> RVADTVGTGPTNSEAIPALTAAETGHTSQVVPGDTMQTRHVKNYHSRSESTIENFLCRSACVYFTEYENSGAKRYAEWVLTPRQAAQLRRKLEFFTYVRFDLELTFVITSTQQPSTTQNQDAQILTHQIMYVPPGGPVPDKVDSYVWQTSTNPSVFWTEGNAPPRMSIPFLSIGNAYSNFYDGWSEFSRNGVYGINTLNNMGTLYARHVNAGSTGPIKSTIRIYFKPKHVKAWIPRPPRLCQYEKAKNVNFQPSGVTTTRQSITTMTN;> GYSDRARSITLGNSTITTQECANVVVGYGVWPDYLKDSEATAEDQPTQPDVATCRFYTLDSVQWQKTSPGWWWKLPDALSNLGLFGQNMQYHYLGRTGYTVHVQCNASKFHQGCLLVVCVPEAEMGCATLDNTPSSAELLGGDSAKEFADKPVASGSNKLVQRVVYNAGMGVGVGNLTIFPHQWINLRTNNSATIVMPYTNSVPMDNMFRHNNVTLMVIPFVPLDYCPGSTTYVPITVTIAPMCAEYNGLRLAGHQ;> GLPTMNTPGSCQFLTSDDFQSPSAMPQYDVTPEMRIPGEVKNLMEIAEVDSVVPVQNVGEKVNSMEAYQIPVRSNEGSGTQVFGFPLQPGYSSVFSRTLLGEILNYYTHWSGSIKLTFMFCGSAMATGKFLLAYSPPGAGAPTKRVDAMLGTHVVWDVGLQS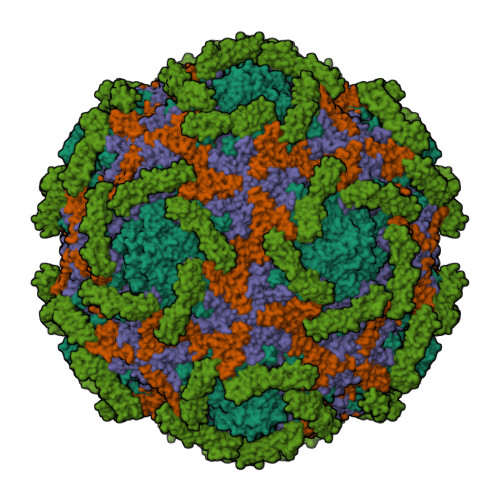SCVLCIPWISQTHYRYVTSDEYTAGGFITCWYQTNIVVPADAQSSCYIMCFVSACNDFSVRLLKDTPFISQQNFFQ;> GAQVSTQKTGAHETGLNASGNSIIHYTNINYYKDAASNSANRQDFTQDPGKFTEPVKDIMIKSLPALN;> CEVPTRLNSASLKQPYITQNYFPVGTVVEYECRPGYRREPSLSPKLTCLQNLKWSTAVEFCKKKSCPNPGEIRNGQIDVPGGILFGATISFSCNTGYKLFGSTSSFCLISGSSVQWSDPLPEC> GAMGSLKISDNEYALIEHPGFANNKDAFFQTLGGVQSIQKACQTSFQNPAAALLELNLRPKDKYHHPVQARVQSRNDLLVTIKKMDNSVQNVSRIRQVFLFRDMADFQYSTQ;> SSNSPSLETDVDDVENIVFQFQNSSLDFQSSDDFSILGIDQPHPIVRIGGMFFRGTWHQPIGTDIVVPSVNDSELSRDGLVLCKRRLMLEQI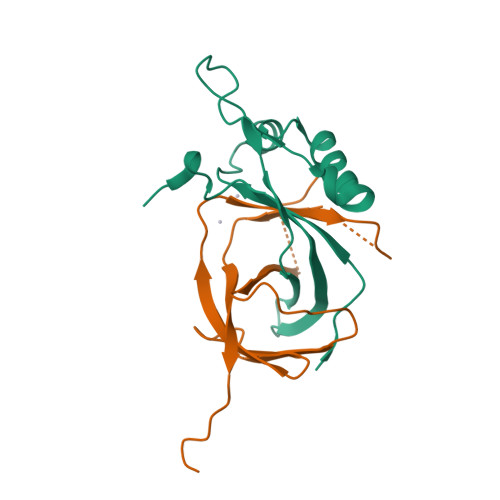RLVPKNPS>MLGAIAYTGNKQSLLPELKSHFPKYNRFVDLFCGGLSVSLNVNGPVLANDIQEPIIEMYKRLINVSWDDVLKVIKQYKLSKTSKEEFLKLREDYNKTRDPLLLYVLHFHGFSNMIRINDKGNFTTPFGKRTINKNSEKRFNHFKQNCDKIIFSSLHFKDVKILDGDFVYVDPPYLITVADYNKFWSEDEEKDLLNLLDSLNDRGIKFGLSNVLEHHGKENTLLKEWSKKYNVKHLNKKYVFNIYHSKEKNGTDEVYIFN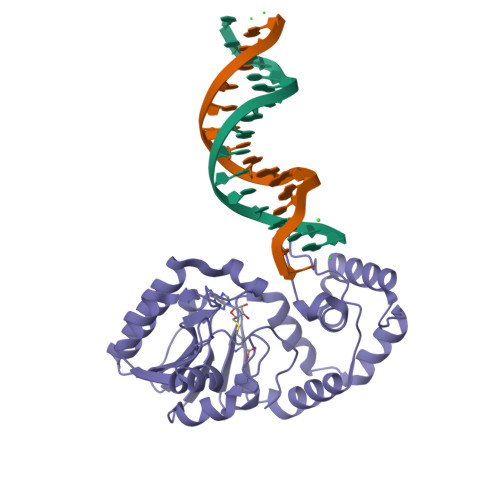[6x]> MARGLVIGEALIDIVDGPDPAEYVGGSPLNVAVGLARLGRDVDLLTHIGRDARGRRIAEYIESSGVQLVSGSQTADRTPTATARIGPDGSATYAFDLEWQIPDTPPVAPPLLVHTGSIAAAREPGCLAVAALLDAYRAAATVSFDPNVRPSLSADPDLTRRRIQRLVERSD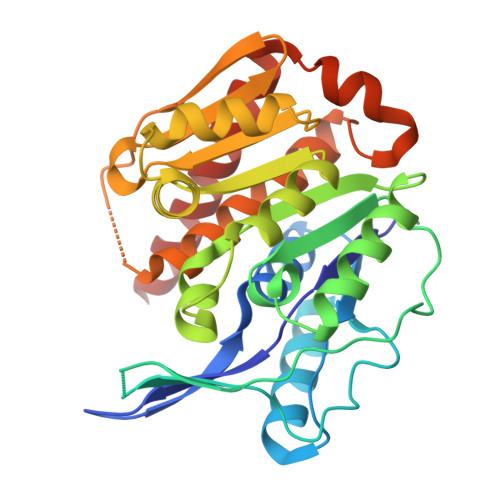IIKASAEDLHWIDPTQPPEQTARAWLACGPAIVALTLGDQGAVAFCAAGPASVPAQPVRVVDTVGAGDAFMAGLLDTLWEQGLLGADRRTELRKIGVSALTSALEVAALTSALTVARAGA> VDFVYRVDSTPPDVIFRDGFSLLGYNRNFQQFISGRSCSGGSSDSRYIATTSSVNQTYAIARAYYSRSTFKGNLYRYQIRADNNFYSLLPSITYLETQGGHFNAYEKTMMRLQREYVSTLSILPENIQKAVALVYDSATGLVKDGVSTMNASYLGLSTTSNPGVIPFLPEPQTYTQQRIDAFGPLISSCFSIG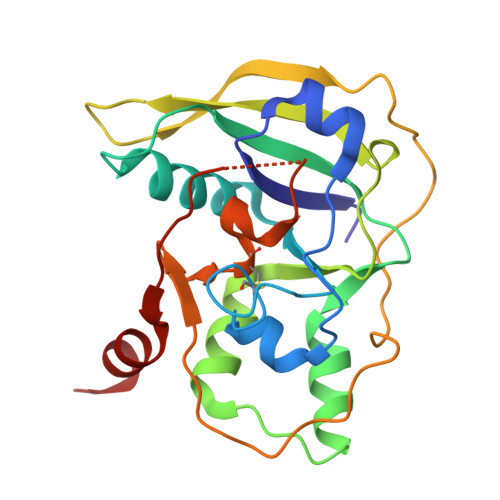SVCHSHRGQRADVYNMSFYDARPVIELILSK>MAPHGDGLSDIEEPEVDAQSEILRPISSVVFVIAMQAEALPLVNKFGLSETTDSPLGKGLPWVLYHGVHKDLRINVVCPGRDAALGIDSVGTVPASLITFASIQALKPDIIINAGTCGGFKVKGANIGDVFLVSDVVFHDRRIPIPMFDLYGVGLRQAFSTPNLLKELNLKIGRLSTGDSLDMSTQDETLIIANDATLKDMEG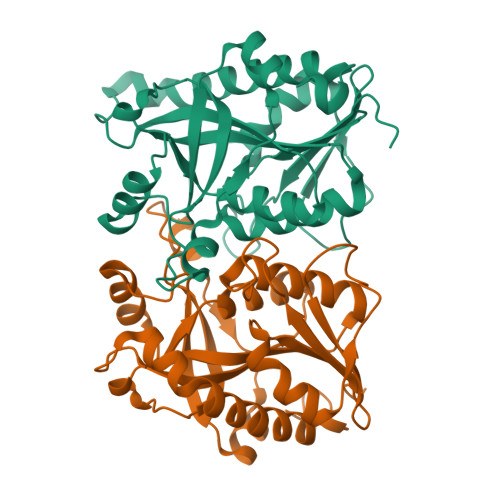AAVAYVADLLKIPVVFLKAVTDLVDGDKPTAEEFLQNLTVVTAALEGTATKVINFINGRNLSDL[2x]> MATDAASAPHSLTFPRGIFAKLSPHPYLLRTLCPDPSNSSSTPQRTNGRRPNEARPFRVNLGSLSHAHGSALVRAGDTTVLCGVRGEVLPVERIPLFRQPDVNGSGIGATVGR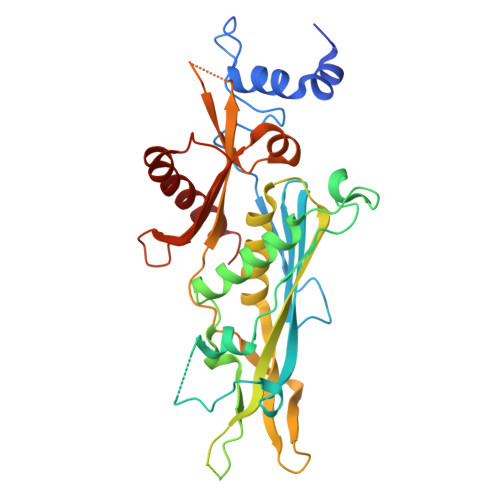GELKEYDLLVPNIELATGSAPQFLPGVPPTALAQTLSTRVYSLLHSTRLVSAEELRIWYRPVATNRSKEGEDVEMEEECQEESGEEQDRVVAYWVLYIDLVFLSFDGNPFDVAWAAVVAALRDTKLPVARWDPDREMVVCSKTETMKLTIKGLPIACSAAVFLEKEHGEVAVGEKNRHWILLDPDRLEESLCKEVITMVVDFSDGETRIRAIEKQGGTVFGRELIRSFALVAEDRWKVVKEVMK The adhesin FimH at the fimbrial tip specifically binds in a catch-bond mode to terminal α-D-linked mannoses of N-linked glycans of the receptor uroplakin 1a on urinary epithelial cells. FimH is a two-domain protein, composed of an N-terminal, mannoside-binding lectin domain (FimHL) and a C-terminal pilin domain (FimHP). FimHP possesses an incomplete immunoglobulin-like fold that is completed by insertion of an N-terminal donor strand of FimG, the subsequent subunit in pilus assembly. The two-domain architecture of FimH is a prerequisite for catch-bond formation because the interactions between FimHL and FimHP determine the conformational state and ligand-binding properties of FimHL.

To test whether ligand-binding causes domain separation in FimH, we determined the co-crystal structure of the ternary complex of FimHF18·DsG with n-heptyl α-D-mannoside (HM), an established model ligand of FimH20, as well as crystal structures of the isolated FimHLF18 and FimHLK12 lectin domains in complex with HM. The isolated lectin domains (residues 1–159) of both FimH variants (FimHLK12 and FimHLF18) were produced by direct expression in the E. coli periplasm and were purified as described. Displacement of GN-FP-4 from FimHL by increasing HM concentrations under equilibrium conditions showed that both FimHLK12 and FimHLF18 bind HM with 3,300-fold higher affinity compared with the respective FimH·DsG complexes (Kd values 1.1 and 3.0 nM, respectively). In an inverse competition experiment, in which HM in preformed FimHL·HM complexes was displaced by GN-FP-4, off-rates of 2.0 × 10−4 and 3.5 × 10−4 s−1 were determined for FimHLK12 and FimHLF18, respectively, corresponding to dissociation half-lives of 58 and 33 min. On the basis of these measured off-rates and equilibrium dissociation constants, kon rates of 1.8 × 105 and 1.2 × 105 M−1 s−1 were calculated for FimHLK12 and FimHLF18, respectively. The on-rates for the isolated FimHL domains are thus 30-fold lower than those of the corresponding full-length FimH·DsG complexes. Previous ligand-binding studies on the isolated FimHL domain mimic the domain-separated Sbound state of FimH. This state is characterized by extremely low off-rates and is promoted in vivo only after ligand-binding and the onset of flow conditions.

>FACKTANGTAIPIGGGSANVYVNLAPAVNVGQNLVVDLSTQIFCHNDYPETITDYVTLQRGSAYGGVLSSFSGTVKYNGSSYPFPTTSETPRVVYNSRTDKPWPVALYLTPVSSAGGVAIKAGSLIAVLILRQTNNYNSDDFQFVWNIYANNDVVVPTG[2x]>[4x]DEPGVATGNGQPVTGNWLAGASQGDGVPIPSQIADQLRGKEFKSWRDFREQFWMAVSKDPSAL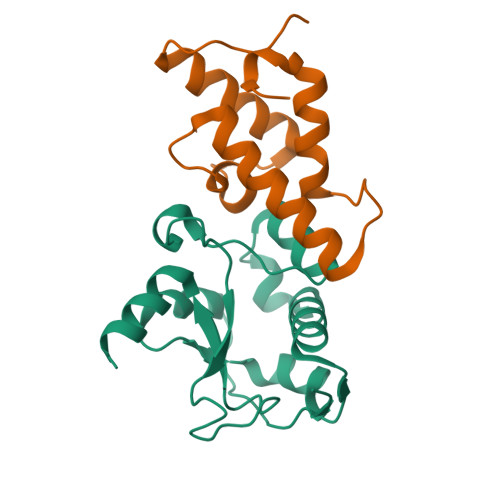ENLSPSNRYFVSQGLAPYAVPEEHLGSKEKFEIHHVVPLESGGALYNIDNLVIVTPKRHSEIHKELKLKRKEK;>[4x]MDIKNNLSDYTESEFLEIIEEFFKNKSGLKGSELEKRMDKLVKHFEEVTSHPRKSGVIFHPKPGFETPEGIVKEVKEWRAANGLPGFKAGLEHHHHHH> MSGSMKEEIKRLAEELKEKTKNEEIKRLAEEAAELAERSDDPEVLEVVKKALEEALKSKNEEKIELLLLVAVLVAEAGSVDAVEEKLEIALLALKLAEESKDPRIIRGALRAAIAALRSDDPLALKTVKEALERARASKDERLIRAILAAAYAFALLA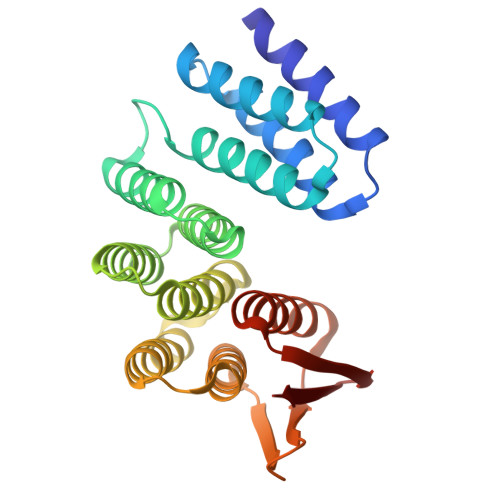VAGASAERLKEAEAIVKELIAAAEKGASPQELVLLVIEMMVKGMGVTMETHRSGNEVKVVIKGLHESQQEVLLEAVLFAAELMGVRVRIRFKGDTVTIVVRE> MPEITRRRALTAAAAVAATASAAVTLAAPAASAAGHHEPAAPESFDEVYKGRRIQGRPAGGGAHHHEHGGGYEVFVDGVQLHVMRNADGSWISVVSHFDPVPTPRAAA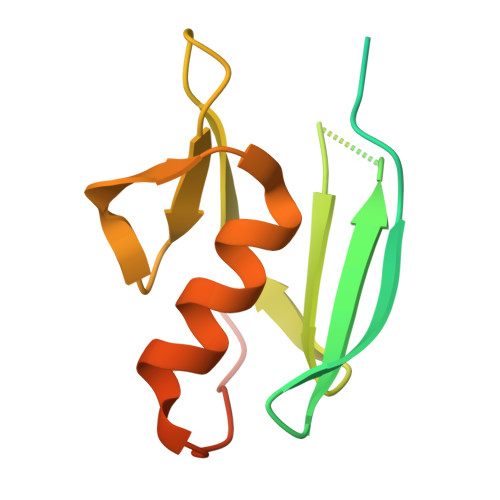RAAVDELQGAPLLPFPANLEHHHHHH> GPGSASCLELALEGERLCKSGDCRAGVSFFEAAVQVGTEDLKTLSAIYSQLGNAYFYLHDYAKALEYHHHDLTLARTIGDQLGEAKASGNLGNTLKVLGNFDEAIVCCQRHLDISRELNDKVGEARALYNLGNVYHAKGKSFGCPGPQDTGEFPEDVRNALQAAVDLYEENLSLVTALGDRAAQGRAFGNLGNTHYLLGNFRDAVIAHEQRLLIAKEFGDKAAERRAYSNLGNAYIFLGEFETASEYYKKTLLLARQLKDRAVEAQSCYSLGNTYTLLQDYEKAIDYHLKHLAIAQELKDRIGEGRACWSLGNAYTALGNHDQAMHFAEKHLEISREVGD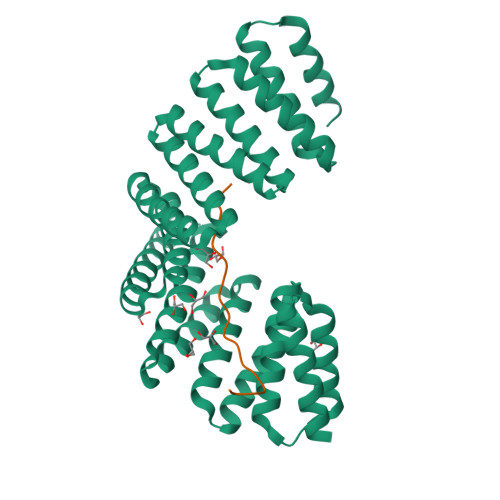;> ALGLLAPLRETKSTNPASRVMEMEPETMETKSVIDSRV>[2x]MASKEIKPIENSIVKEIIV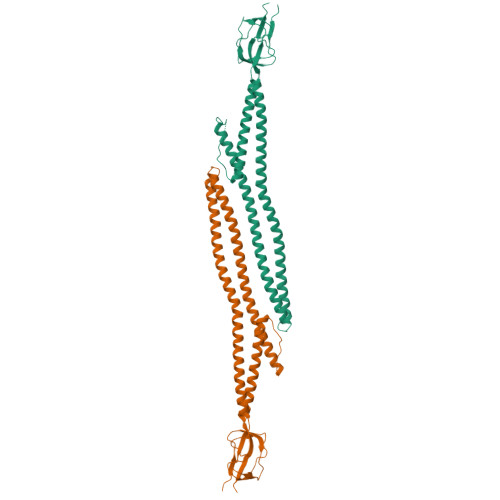KEGESVRKGDVLLKLTALGAEADTLKTQSSLLQTRLEQTRYQILSRSIELNKLPELKLPDEPYFQNVSEEEVLRLTSLIKEQFSTWQNQKYQKELNLDKKRAERLTILARINRYENLSRVEKSRLDDFRSLLHKQAIAKHAVLEQENKYVEAANELRVYKSQLEQIESEILSAKEEYQLVTQLFKNEILDKLRQTTDNIELLTLELEKNEERQQASVIRAPVSGKVQQLKVHTEGGVVTTAETLMVIVPEDDTLEVTALV>MSADVAGAVIDGAGLGFDVLKTVLEALGNVKRKIAVGIDNESGKTWTAMNTYFRSGTSDIVLPHKVAHGKALLYNGQKNRGPVATGVVGVIAYSMSDGNTLAVLFSVPYDYNWYSNWWNVRVYKGQKRADQRMYEELYYHRSPFRGDNGWHSRGLGYGLK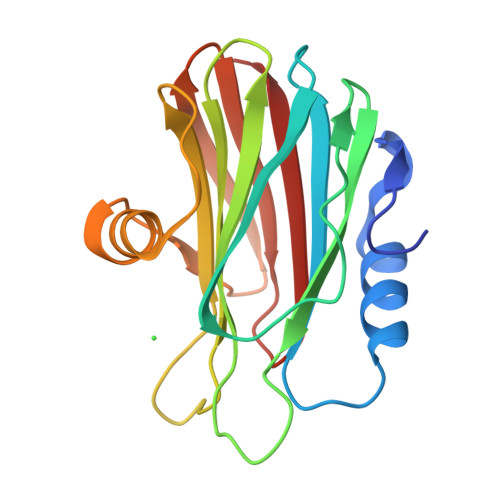SRGFMNSSGHAILEIHVTKA[4x]>[3x]DPSLNNPVVIQATRLDASILPRNVFSKSYLLYVIAQGTDVGAIAGKANEAGQGAYDAQVKND;>[6x]PIQQLPMMKGMGKDFKNADYIDYLPVNMLATPKEILNSSGYLRSFPGITKRYDMNGVSRGVEYNTAQNAVYRVCGGKLYKGESEVGDVAGSGRVSMAHGRTSQAVGVNGQLVEYRYDGTVKTVSNWPADSGFTQYELGSVRDITRLRGRYAWSKDGTDSWFITDLEDESHPDRYSAQYRAESQPDGIIGIGTWRDFIVCFGSSTIEYFSLTGATTAGAALYVAQPSLMVQKSIAGTYCKTPFADSYAFISHPATGAPSVYIIGSGQASPIATASIEKIIRSYTAEEMATGVMETLRFDSHELLIIHLPRHVLVYDASSSQNGPQWCVLKTGLYDDVYRGVDFMYEGNQITCGDKSEAVVGQLQFDISSQYDKQQEHLLFTPLFKADNARCFDLEVESSTGVAQYADRLFLS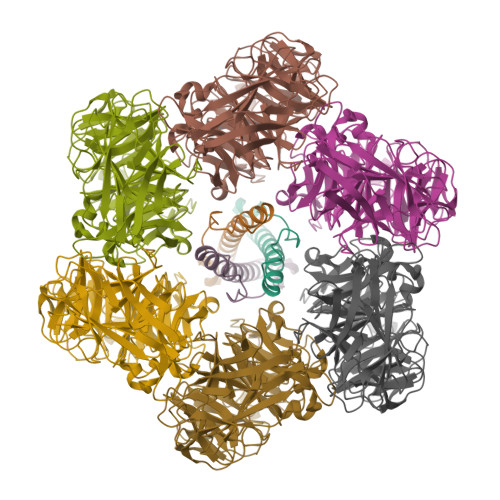ATTDGINYGREQMIEQNEPFVYDKRVLWKRVGRIRRLIGFKLRVITKSPVTLSGCQIRLE~{N}-[2-(3,4-dichlorophenyl)-3,4-dihydropyrazol-5-yl]ethanamide | C11 H11 Cl2 N3 O | 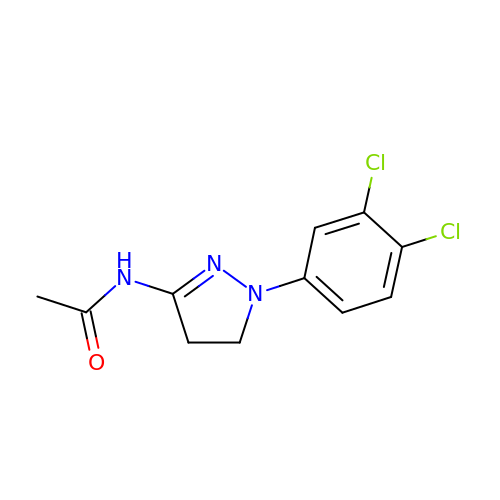CQPBYZABXGBFMI-UHFFFAOYSA-N>[3x]MNMDWALFLTFLAACGAPATTGALLKPDEWYDNLNKPWWNPPRWVFPLAW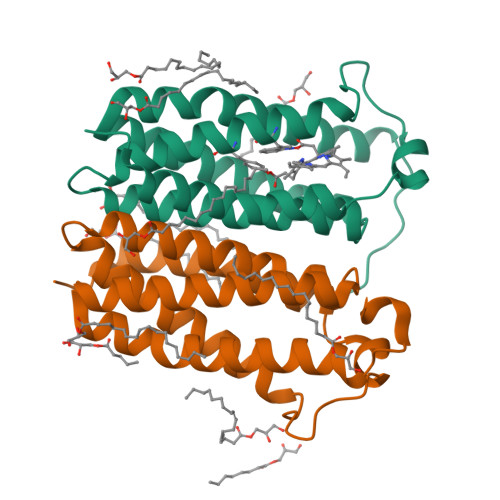TSLYFLMSLAAMRVAQLEGSGQALAFYAAQLAFNTLWTPVFFGMKRMATALAVVMVMWLFVAATMWAFFQLDTWAGVLFVPYLIWATATTGLNFEAMRLNWNRPEAR> GFDPEKAQCCLVENGQILTHGSGGKGYGLASTGVTSGCYQWKFYIVKENRG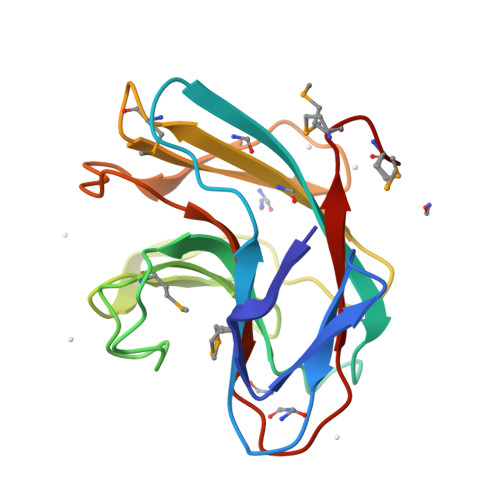NEGTCVGVSRWPVHDFNHRTTSDMWLYRAYSGNLYHNGEQTLTLSSFTQGDFITCVLDMEARTISFGKNGEEPKLAFEDVDAAELYPCVMFYSSNPGEKVKICDMQMR>GSHMTDRTDADDL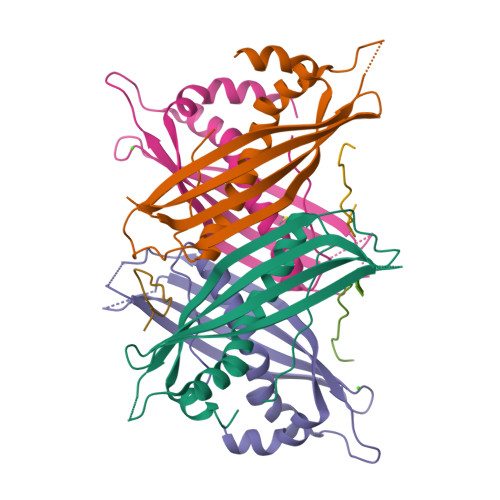DLQRVGARLAARAQIRDIRLLRTQAAVHRAPKPAQGLTYDLEFEPAVDADPATISAFVVRISCHLRIQNQAADDDVKEGDTKDETQDVATADFEFAALFDYHLQEGEDDPTEEELTAYAATTGRFALYPYIREYVYDLTGRLALPPLTLEILSRPMPVSPGAQWPATRGTP[4x];>EVPTWHRLSSYRG[3x]> MKIIKDKVAKLSFVALLVTVTAAMFYTPTASAHGEKSQAAFMRMRTIHWFDLNWSKDQVSVNETMSISGKFHVFAGWPETVDKPEVAFLNIGIPGPVFIRAGSWIGGQLVPRSVSLELGETYEFKVLLKARRPGDWHVHTMMNVQGGGPIIGPGKWVTITGSMGDFKNPITTLTGETIDLETYALDGVYGWHLFWYLLGVAWMVYWCRKPVFIPRRIAVDAGKADSLITPTDKKVGMAFAAGTLAIVAVSMGQANEKYPVTTPLQAGLMRGIKSLELPQPTVSVKVVDASYRVPGRAMQMTLEITNNGDSAVRLAEFNTASVRFLDADVYEDDTNYPDDLLAEEGLSVSDNSPLAPGETRTVDVTASDAAWEVYRLADLIYDPDSRFAGLLFFIDEDGNRQMTMVDAPLIPTFI;> MSASQSAVRSRAEAVKVSRTFDYMILFTVFFVVLGGYHIHYMLTGGDWDFWTDWKDRRLWVTVAPIVSITFPAAVQAVLWWRYRIAWGATLCVLGLLLGEWINRYFNFWGWTYFPVNFVFPSNLMPGAIVLDVILMLSNSMTLTAVVGGLAWGLLFYPGNWPIIAPLHVPVEYNGMMMTLADLQGYHYVRTGTPEYIRMVEKGTLRTFGKDVAPVSAFFSGFVSILIYFLWHFFGSWFGSEKFVQAA;> MAATTESVKADAAEAPLLNKKNIIAGASLYLVFYAWVRWYEGVYGWSAGLDSFAPEFETYWMNFLYIEMVLEVLTASVLWGYIWKSRDRKVMSITPREEL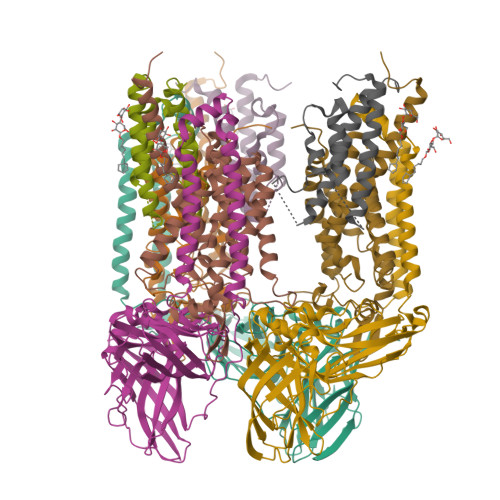RRHFTHWTWLMMYGIAIYFGASYFTEQDGTWHQTIVRDTDFTPSHIIEFYLSYPIYIITGGASFLYAKTRLPTYQQGLSLQYLVVVVGPFMILPNVGLNEWGHTFWFMEELFVAPLHYGFVFFGWSALGVLGVINIELGALSKLLKKDLA>MAEAEAGGDEARCVRLSAERAKLLLAEVDTLLFNCDGVLWRGETAVPGAPETLRALRARGKRLGFITNNSSKTRTAYAEKLRRLGFGGPVGPEAGLEVFGTAYCSALYLRQRLAGVPDPKAYVLGSPALAAELEAVGVTSVGVGPDVLHGDGPSDWLAVPLEPDVRAVVVGFDPHFSYMKLTKAVRYLQQPDCLLVGTNMDNRLPLENGRFIAGTGCLVRAVEMAAQRQADIIGKPSRFIFDCVSQEYGINPERTVMVGDRLDTDILLGSTCSLKTILTLTGVSSLEDVKSNQESDSMFKKKMVPDFYVDSIADLLPALQG[2x]

Phosphoglycolate phosphatase (PGP, also called glycerol 3-phosphate phosphatase or AUM11) is an evolutionarily conserved metabolite damage control enzyme that can dephosphorylate and thereby repair three adventitious glycolytic metabolites: 2-phospho-L-lactate, 4-phosphoerythronate, and 2-phosphoglycolate. PGP belongs to the haloacid dehalogenase (HAD)-type superfamily of phosphatases, a large, widespread and evolutionarily ancient class of hydrolases with emerging roles in human physiology and disease. All HAD phosphatases consist of a catalytic core domain with a Rossmanoid-fold. This core is accessorized with so-called cap domains, which are mobile elements that can shield the entry to the catalytic cleft.

CP1-bound PGP crystallized in the tetragonal space group P41 with one dimer per asymmetric unit. CP1 binds adjacent to, but not directly into, the PGP active site with one of the benzoic acid moieties (referred to in the following as proximal) at a distance of just below 6 Å from the catalytic Asp34 (Asn34). The proximal benzoic acid moiety of CP1 forms the only direct hydrogen bonds via its carboxylic acid to the nitrogen atom of the carboxamide function of Asn199 and to the side chain hydroxyl group of Thr215. Overall, CP1 is embedded in a cavity that extends from the active site of monomer A towards the dimerization interface with monomer B. One side of this cavity is formed by the more polar residues 35–37, 68–71, 125–127 and 143–145, which originate entirely from monomer A. In contrast, the opposite side is formed by both monomers and is generally more hydrophobic in character. Domain movements were recognized for both subunits of the inhibitor-bound structure only with respect to chains D and E of the apo-structure, thus indicating that both monomers of the CP1-bound structure and the majority of apo-PGP monomers adopt the same conformational state. Despite being in the same conformational state, there are differences between the closed state in the apo and inhibitor bound structures, e.g. the substrate binding loop, rather than moving solely towards the active site, is also translated outwards. This additional movement is needed to create the space required for incorporating CP1. Hence, CP1 appears to inhibit PGP activity by locking it in a cap-closed conformation. Based on the inhibitor-bound structure and the competitive component of PGP inhibition by CP1 (increased KM), it seems likely that CP1 sterically hinders substrate access to the active site. In addition, the cap-closed conformation of CP1-bound PGP will block solvent entry into the enzymatic pocket, and thus prevent the hydrolysis of the phospho-aspartate intermediate during the final catalytic step.> AIASEFSSLPSYAAYATAQEAYEQAVANGDSEVVLKKLKKSLNVAKSEFDRDAAMQRKLEKMADQAMTQMYKQARSEDKRAKVTSAMQTMLFTM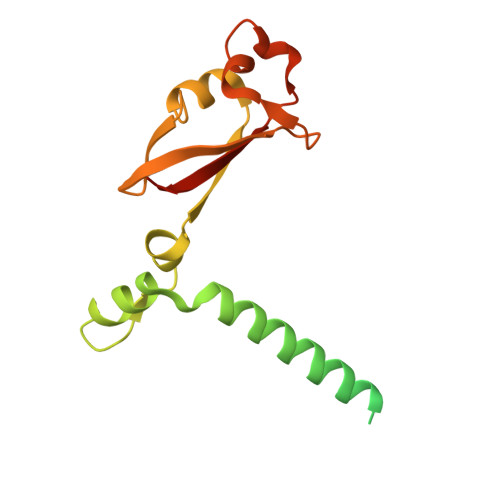LRKLDNDALNNIINNARDGCVPLNIIPLTTAAKLMVVVPDYGTYKNTCDGNTFTYASALWEIQQVVDADSKIVQLSEINMDNSPNLAWPLIVTALRANSAVKLQ> MCPRAARAPATLLLALGAVLWPAAGAWELTILHTNDVHSRLEQTSEDSSKCVDASRCMGGVARLFTKVQQIRRAEPNVLLLDAGDQYQGTIWFTVYKGAEVAHFMNALRYDAMALGNHEFDNGVEGLIEPLLKEAKFPILSANIKAKGPLASQISGLYLPYKVLPVGDEVVGIVGYTSKETPFLSNPGTNLVFEDEITALQPEVDKLKTLNVNKIIALGHSGFEMDKLIAQKVRGVDVVVGGHS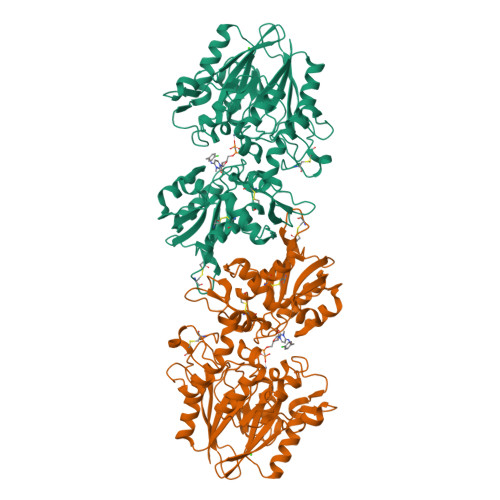NTFLYTGNPPSKEVPAGKYPFIVTSDDGRKVPVVQAYAFGKYLGYLKIEFDERGNVISSHGNPILLDSSIPEDPSIKADINKWRIKLDDYSTQELGKTIVYLDGSSQSCRFRECNMGNLICDAMINNNLRHTDEMFWNHVSMCILNGGGIRSPIDERNDGTITWENLAAVLPFGGTFDLVQLKGSTLKKAFEHSVHRYGQSTGEFLQVGGIHVVYDLSRKPGDRVVKLDVLCTKCRVPSYDPLKMDEVYKVILPNFLANGGDGFQMIKDELLRHDSGDQDINVVSTYISKMKVIYPAVEGRIKFSGGGGAGGGGGTKHHHHHH>MQI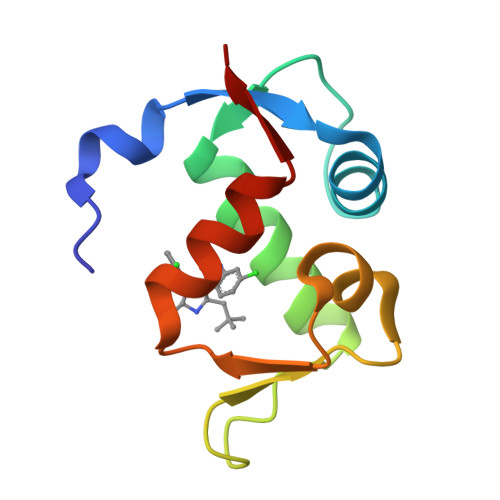PASEQETLVRPKPLLLKLLKSVGAQKDTYTMKEVLFYLGQYIMTKRLYDEKQQHIVYCSNDLLGDLFGVPSFSVKEHRKIYTMIYRNLVVVN[3x]>MDLFPEKNESNPQAEDEPTATVCDRWGSRDVAGGRYRVINNVWGAETAQCIEIGLETGNFILTRAEHSNGDNVAAYPAIYLGCHWGACTSQSGLPLRVEAISRLQSNWRLTPISSGRWNAAYDLWFS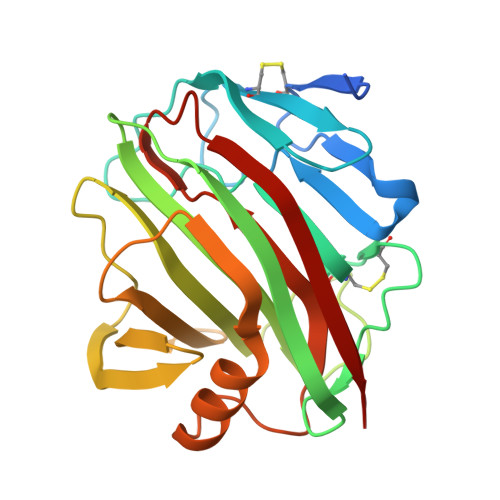PSLTSTNGYSGGAELMIWLNWRGNVMPGGNRVATVSLAGATWEVWFADWDWNYIAYRRTTPVTEVTQLDLKAFIDDAVARGYISPTWYLHAVETGFELWEGGRGLKSSDFSVTLTAR[2x]> MDTWKVGPVELKSRLILGSGKYEDFGVMREAIAAAKAEVVTVSVRRVELKAPGHVGLLEALEGVRLLPNTAGARTAEEAVRLARLGRLLTGERWVKLEVIPDPTYLLPDP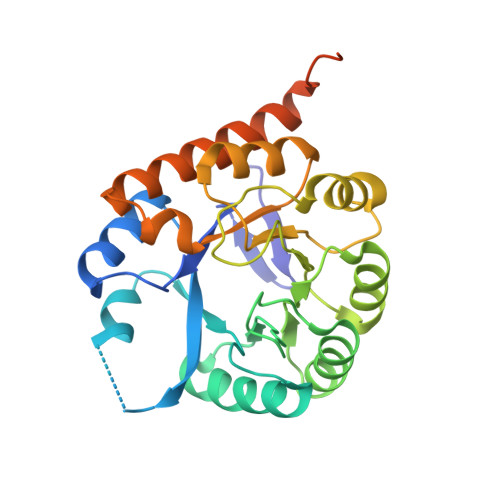LETLKAAERLIEEDFLVLPYMGPDLVLAKRLAALGTATVMPLAAPIGSGWGVRTRALLELFAREKASLPPVVVDAGLGLPSHAAEVMELGLDAVLVNTAIAEAQDPPAMAEAFRLAVEAGRKAYLAGPMRPREAASPSSPVEGVPFTPTGPRPGRGPQ> VVNGIPTRTNIGWMVSLRYRNKHICGGSLIKESWVLTARQCFPSRDLKDYEAWLGIHDVHGRGDEKCKQVLNVSQLVYGPEGSDLVLMKLARPAVLDDFVSTIDLPNYGSTIPEKTSCSVYGWGYTGLINYDGLLRVAHLYIMGNEKCSQHHRGKVTLNESEICAGAEKIGSG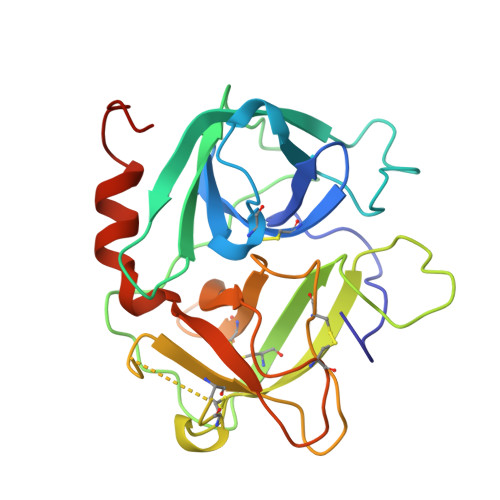PCEGDYGGPLVCEQHKMRMVLGVIVPGRGCAIPNRPGIFVRVAYYAKWIHKIILTYKVPQSHHHHHH> MAYDDLHEGYATYTGSGYSGGAFLLDPIPSDMEITAINPADLNYGGVKAALAGSYLEVEGPKGKTTVYVTDLYPEGARGALDLSPNAFRKIGNMKD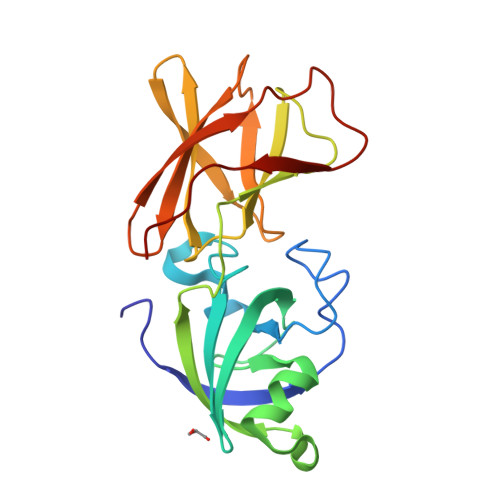GKINIKWRVVKAPITGNFTYRIKEGSSRWWAAIQVRNHKYPVMKMEYEKDGKWINMEKMDYNHFVSTNLGTGSLKVRMTDIRGKVVKDTIPKLPESGTSKAYTVPGHVQFPE>[2x]GASCDKFDEINTDPDATTKVTSSLLATGLLLDITSSSASKSFIYDELLAKQMAWGE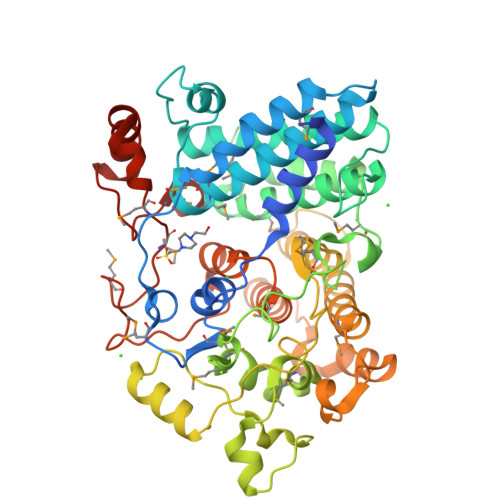SMEDYQYNVFGRSGFGGYTTLINAQKMVESVSDDNVNAYDGLAHFIKAYKIFYMSMEMGDLPYEEALQGELGLVRPKYNTQKEVMNFILSDLETAYELFSTAKDFDGDPILGGSISKWKKATTAFQLKVLMHLSKKESDADLKVKERFARIVASGSLMESNEDNLQMKYADKANTVYPFHNTNTKHAGYAMLSTMLIDKFKATGDIRMFYYAKPAKAKLNEGVTADSWDAYIGTDPSLPFEQIEKAYATEQYSGFNARYTDYPSGEPVVRLGYAEQNFILAEAAVRGWISGDASAYYKKAIRAHMEFIASNTPDEEVYHHGHPITEEAIAAFLETPAIQLSGEKEEDIEKILTQRYLASFMQHPYDVYYDYRRTGYPVLPINPATNRNTMNDRLPMRWMYPKSESDYNLEHQNEALERQFGGVDDVNKLMWILQ> GPLGSPEFMINGVSLQGTAGYEAHTEEGNVNVKKLLESLNSKSLGDMDKDSELAATLQKMINPSGGDGNCSGCALHACMAMLGYGVREAPVPNEISEYMTGFFHRHLEQIDSEGI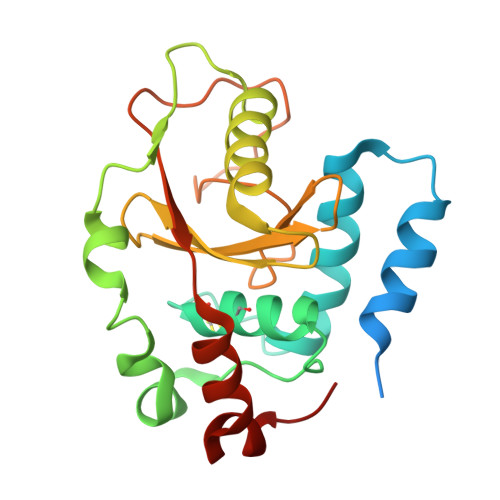VSHPNETYSKFRERIAENILQNTSKGSVVMISIEQATHWIAGFNDGEKIMFLDVQTGKGFNLYDPVEKSPDAFVDENSSVQVIHVSDQEFDHYANSSSWKSKRLC> SQARVSDVEEQVNQYLSKVPELEQKQNVSELLSLLSNSPNISLSQLKAYLEGKSEEPSEQFKMLCGLRDALKGRPELAHLSHLVEQALVSMAEEQGETIVLGARITPEAYRESQSGVNPLQPLRDTYRDAVMGYQGIYAIWSDLQKRFPNGDIDSVILFLQKALSADLQSQQSGSGREKLGIVISDLQKLKEFGSVSDQVKGFWQFFS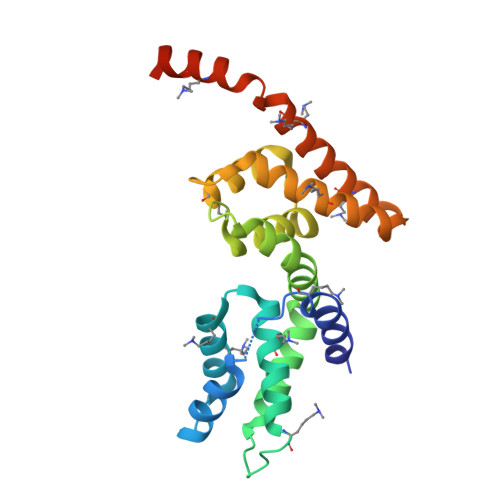EGKTNGVRPF>PNVAIIVAALKPALGIGYKGKMPWRLRKEIRYFKDVTTRTTKPNTRNAVIMGRKTWESIPQKFRPLPDRLNIILSRSYENEIIDDNIIHASSIESSLNLVSDVERVFIIGGAEIYNELINNSLVSHLLITEIEHPSPESIEMDTFLKFPL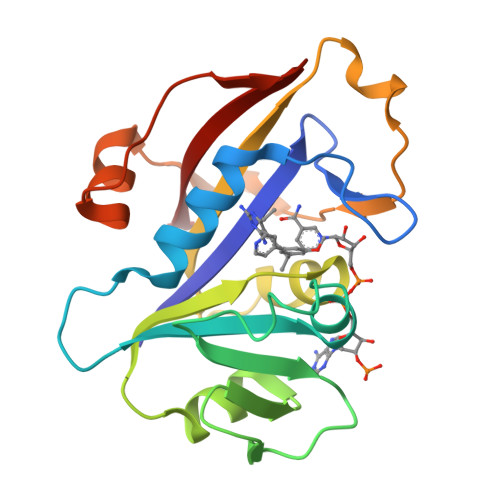ESWTKQPKSELQKFVGDTVLEDDIKEGDFTYNYTLWTRK[2x]> VFPSNATFGMGDRVRKKSGAAWQGQIVGWYCTNLTPE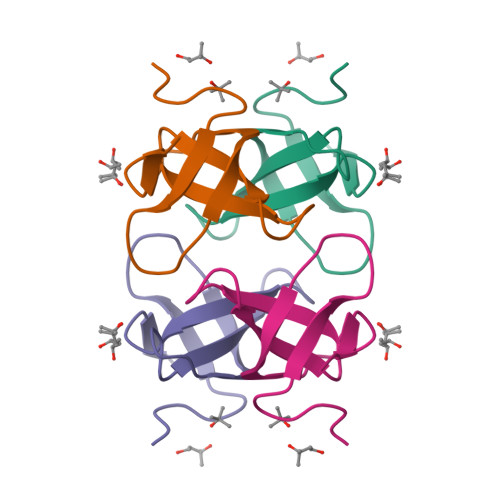GYAVESEAHPGSVQIYPVAALERIN> HHAADYVLYKDATKPVEDRVADLLGRMTLAEKIGQMTQIERLVATPDVLRDNFIGSLLSGGGSVPRKGATAKEWQDMVDGFQKACMSTRLGIPMIYGIDAVHGQNNVYGATIFPHNVGLGATRDPYLVKRIGEATALEVRATGIQYAFAPCIAVCRDPRWGRCYESYSEDRRIVQSMTELIPGLQGDVPKDFTSGMPFVAGKNKVAACAKHFVGDGGTVDGINENNTIINREGLMNIHMPAYKNAMDKGVSTVMISYSSWNGVKMHANQDLVTGYLKDTLKFKGFVISDYEGIDRITTPAGSDYSYSVKASILAGLDMIMVPNKYQQFISILTGHVNGGVIPMSRIDDAVTRILRVKFTMGLFENPYADPAMAEQLGKQEHRDLAREAARKSLVLLKNGKTSTDAPLLPLPKKAPKILVAGSHADNLGYQCGGWTIEWQGDTGRTTVGTTILEAVKAAVDPSTVVVFAENPDAEFVKSGGFSYAIVAVGEHPYTETKGDNLNLTIPEPGLSTVQAVCGGVRCATVLISGRPVVVQPLLAASDALVAAWLPGSEGQGVTDALFGDFGFTGRLPRTWFKSVDQLPMNVGDAHYDPLFRLGYGLTTNATKKY

In the barley β-d-glucan glucohydrolase, a glycoside hydrolase family 3 (GH3) enzyme, the Trp286/Trp434 clamp ensures β-d-glucosides binding, which is fundamental for substrate hydrolysis during plant growth and development. HvExoI folds into a two-domain structure consisting of an (α/β)8 barrel (domain 1) and an (α/β)6 sandwich (domain 2) with a 13 Å-deep active site pocket embracing the subsites −1 and +1, positioned at the interface between the two domains. HvExoI catalyses the hydrolytic removal of nonreducing glucose (Glc) moiety from a broad spectrum of poly- and oligomeric β-d-glucosides. The crucial role of substrate binding in HvExoI implies a pair of the aromatic Trp286 and Trp434 residues that form a clamp at the +1 subsite, which is positioned next to a pocket-shaped site at the −1 subsite, housing the Asp285 and Glu491 catalysts.

To find out, if the Glc molecule alone adopts similar or different dispositions at the −1 and +1 subsites, we perfused Glc into WT, W434A, and W286Y, and compared their positions, which at the −1 subsite were identical in all instances, but at the +1 subsite of W434A the Glc molecule was disordered (data not shown). The Glc molecule entrapped in the −1 subsite is held at the bottom of the pocket by at least 10 residues. Notable was the behaviour of W286Y that showed increased catalytic efficiency values with (1,3;1,6)-β-d-glucan (laminarin), laminaribiose (G3OG), and 4NP-Glc, while these values in W434Y were considerably lower.>EAEAAASANDISFNFQRFNETNLILQGDASVSSSGQLRLTNLNDNGEPTLSSLGRAFYST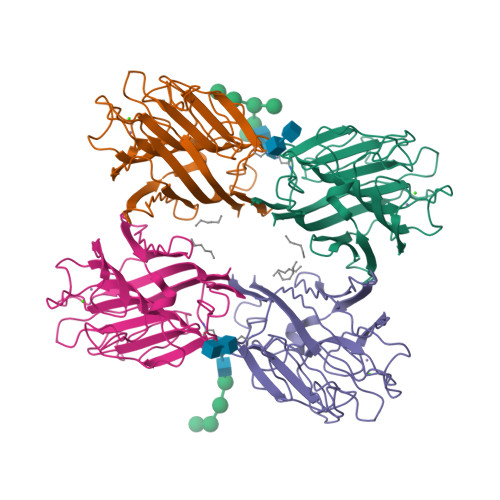PIQIWDSTTGAVASFATSFTFNIRVPNNAGPADGLAFALVPVGSKPKDRGGLLGLFDGSDSKAHTVAVEFDTLYNRDWDPRERHIGIDVNSIKSIKTTPWDFVNGEDAEVLITYDSSTKLLVASLVYPSQKTSFIVSDTVDLKSVLPEWVSVGFSATSGISKGNVETNDLLSWSFASKLSDGTTSEGLNHHHHHH[4x]>[4x]SMEDQEENTLRELRLFLRDVTKRLATDKRFNIFSKPVDIEEVSDYLEVIKEPMDLSTVITKIDKHNYLTAKDFLKDIDLICSNALEYNPDKDPGDKIIRHRACTLKDTAHAIIAAELDPE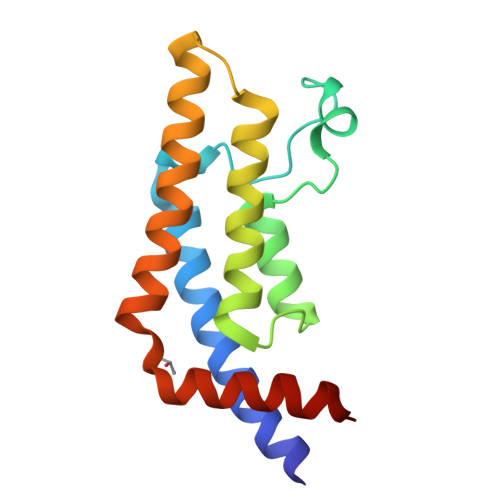FNKLCEEIKEARIKRG>MERVPSAAFASDNAAPAHPRVLEALHHVNQGPAPSYGDDPVTAEAAEALRTAFESPGADVLF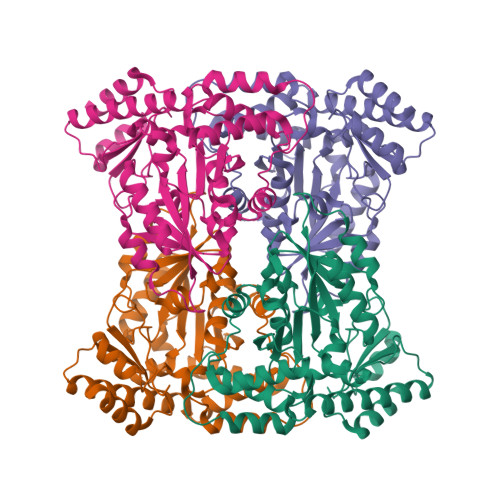AFTGTAANIIALASAVRPWHEIFCSDVAHVLVDEAGGPVRLSGAQLTRLASDDGLISPDELERRVRGRSAVHHSQPRIVSITQSTENGRVWSATAVAQFVDRAHALGLLVHVDGARIANAVAALSISPLEAIGDADIVSVGGTKNGLMFGDAILVRRPAHFDGIHFVQKQIGHLASKHRFVAAQFAGLFEGGLWLRNAAHANAMARRLSTGLEALGLQLASPTESNEVFVKLDGEAHRRLAERYLVHQPDPGQPVVRFVCSWSTTETEVDDALAALRSAGN[4x]>[2x]GARSSSYSGEYGSGGGKRFSHSGNQLDGPITALRVRVNTYYIVGLQVRYGKVWSDYVG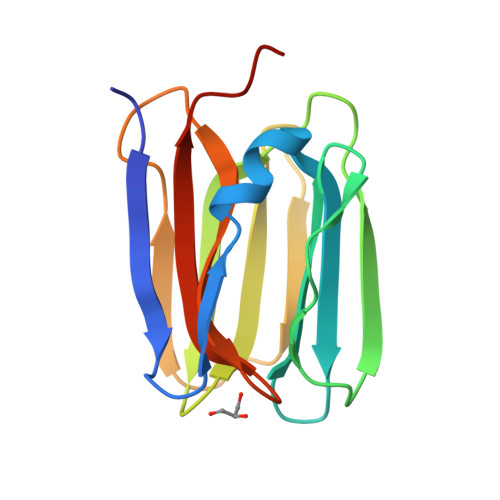GRNGDLEEIFLHPGESVIQVSGKYKWYLKKLVFVTDKGRYLSFGKDSGTSFNAVPLHPNTVLRFISGRSGSLIDAIGLHWDVYPTSCSRC>[10x]SNAMEIIPIPADSYTLGFIGAGKMAESIAKGAVRSGVLSPSRIKTAIHSNPARRTAFESIGITVLSSNDDVVRDSNVVVFSVKPQLLKDVVLKLKPLLTKDKLLVSVAAGIKMKDLQEWAGHERFIRVMPNTAATVGEAASVMSLGGAATEEDANLISQLFGSIGKIWKADDKYFDAITGLSGSGPAYIYLAIEALADGGVAAGLPRDLALSLASQTVLGAASMATQSGKHPGQLKDDVTSP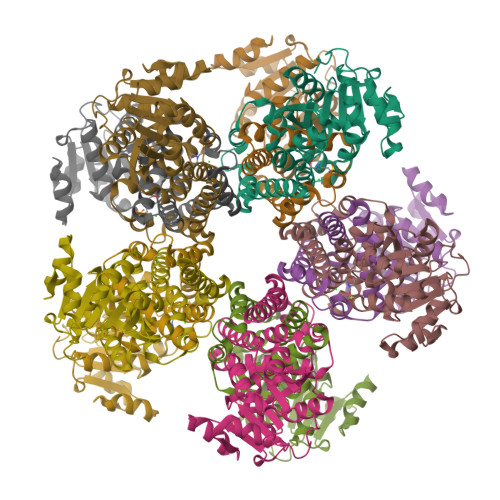GGTTIAGVHELEKAGFRGILMNAVVAAAKRSQELS The Roquin protein is essential in T cells for the prevention of autoimmune disease. We have recently reported structural and functional data of the Roquin-1 ROQ domain bound to a canonical constitutive decay element (CDE), a short stem loop (SL) that acts as a cis-regulatory RNA element in the 3′-untranslated regions (3′-UTRs) of target genes such as Tnf. The ROQ domain adopts an extended winged helix fold that engages predominantly non-sequence-specific protein–RNA contacts and mainly recognizes the shape of the canonical Tnf CDE RNA. Here we present structural and functional evidence for a greatly expanded repertoire of RNA elements that are regulated by Roquin as demonstrated with a novel U-rich hexaloop SL in the 3′-UTR of Ox40 bound to the Roquin-1 ROQ domain.

The structures of ROQ bound to the 20-mer ADE SL and to the 22-mer Ox40 ADE-like SL RNAs were refined to a resolution of 3.0 and 2.2 Å, respectively. Given their highly similar binding modes we focus the following discussion on the structure of the Ox40 ADE-like SL RNA, as it naturally exists in the Ox40 3′-UTR and was solved at higher resolution. Notably, the U-rich hexaloop in the Ox40 ADE-like SL RNA binds to an extended surface on the ROQ domain that cannot be accessed by the CDE triloop11 and includes a few pyrimidine-specific contacts. For example, the main chain atoms of Phe255 form two hydrogen bonds with the Watson–Crick face of the U11 base. The side chain of Lys259 forms hydrogen bonds with the phosphate groups of U10 and U11 and the hydrophobic side chain of Val257 stacks with the U11 base. The RNA stem is closed by a Watson–Crick base pair (C8–G15 in the hexaloop SL RNA). Interestingly, the G9 base stacks on top of this closing base pair and takes a position that is very similar to the purine base of G12 in the CDE triloop. The G9 base does not form a base pair with A14 but rather the A14 base packs into the minor groove of the RNA duplex. This arrangement provides an extended stacking interaction of G9, U10 and Tyr250 in the ROQ domain at the 5′-side of the RNA stem. The preference for U-rich hexaloops depends on nucleotide-specific interactions of ROQ with U10, U11 and U13 in the Ox40 ADE-like SL.

>EEEGRIRAMRAARSLGERTVTELILQHQNPQQLSSNLWAAVRARGCQFLGPAMQEEALKLVLLALEDGSALSRKVLVLFVVQRLEPRFPQASKTSIGHVVQLLYRASCFKVTKRDEDSSLMQLKEEFRTYEALRREHDSQIVQIAMEAGLRIAPDQWSSLLYGDQSHKSHMQSIIDKLQT[2x]(2S)-2-amino-5-[[4-[(2S)-2-hydroxy-2-phenyl-ethoxy]phenyl]amino]-5-oxo-pentanoic 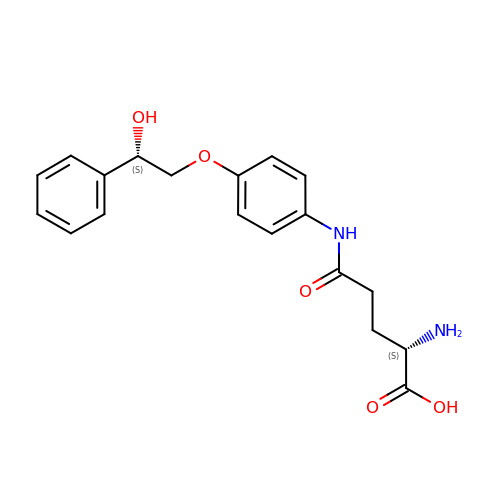acid | C19 H22 N2 O5 | HHPPMARBWOSMFL-DLBZAZTESA-N> MAHSRASTKVVVVGGGGTIGSSTALHLIRSGYTPSNITVLDVYKTPSLQSAGHDLNKIMGIRLRNGPDLQLSLESLDMWQNDELFKPFFHQVGMIDCSSSKEGIENLRRKYQTLLDAGIGLEKTNVWLESEDEILAKAPNFTREQVKGWKGLFCTDGGWLAAAKAINAIGIFLQDKGVKFGFGGAGTFQQPLFAADGKTCIGLETTDGTKYFADKVVLAAGAWSPTLVDLEDQCVSKAWVFAHIQLTPKEADAYKNVPVVYDGEYGFFFEPNEYGVIKVCDEFPGFSRFKLHQPYGAASPKMISVPRSHAKHPTDTYPDASEVTIRKAIARFLPEFKDKELFNRTMCWCTDTADANLLICEHPKWKNFILATGDSGHSFKLLPNIGKHVVELLEGSLSQEMAGAWRWRPGGDALRSRRGAPAKDLAEMPGWK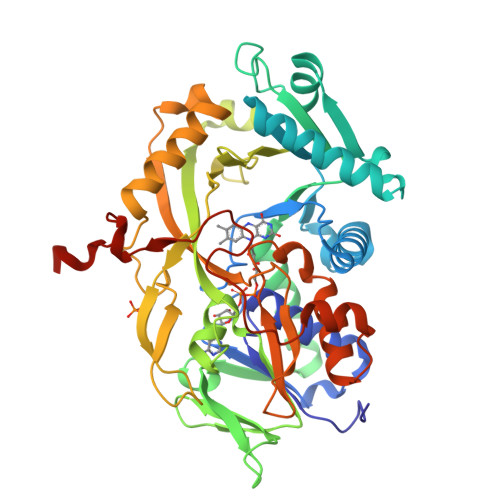HDAHLLEHHHHHH Vimseltinib | C23 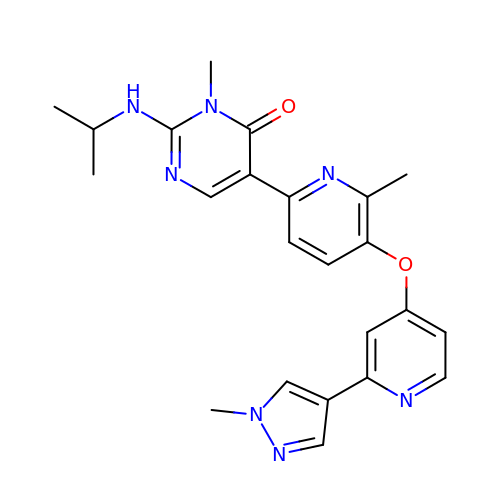H25 N7 O2 | TVGAHWWPABTBCX-UHFFFAOYSA-N> SMRVDYLVTEEEINLTRGPSGLGFNIVGGTDQQYVSNDSGIYVSRIKENGAAALDGRLQEGDKILSVNG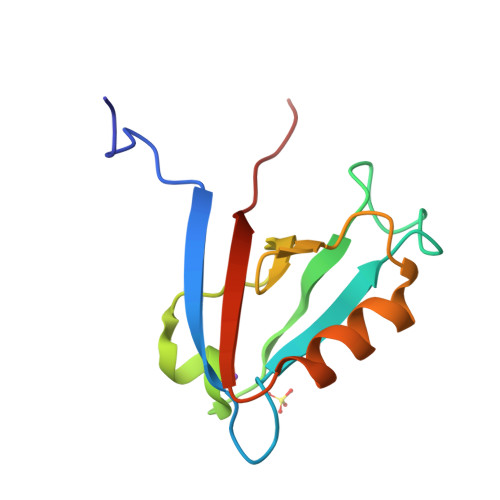QDLKNLLHQDAVDLFRNAGYAVSLRVQHRESSI CLC-7 is a member of the CLC family of chloride (Cl-) channels and chloride (Cl-)/proton (H+) transporters and is expressed in the lysosome and the resorption lacuna of osteoclasts. In the membranes of these acidic compartments, CLC-7 uses the large pH gradient to catalyze the uptake of two Cl- ions for each H+ released. Unique among mammalian CLC transporters, CLC-7 requires a β-subunit, osteopetrosis-associated transmembrane protein 1 (OSTM1), for transport activity. In this study, we present structures of the lysosomal Cl-/H+ exchanger CLC-7 alone and in complex with its obligatory β-subunit OSTM1.

Reconstruction of these particle images with two-fold symmetry imposed yielded a structure of CLC-7 in complex with OSTM1 at a resolution of 2.8 Å. The luminal domains of OSTM1 form a dimeric cap-like structure that covers the luminal surface of CLC-7 while the transmembrane helices pack against the periphery of the CLC-7 transmembrane domain. The luminal domain of OSTM1 is composed of two three-helix bundles. Connecting both within and between the helical bundles are five disulfide bonds that constrain the organization of the luminal domain. At the periphery of the luminal domain, non-protein densities were resolved extending from seven exposed asparagine residues (93, 128, 163, 184, 194, 263 and 274) on OSTM1. Because CLC-7 lacks any N-linked glycosylation sites, the glycosylation shell surrounding the rigid, disulfide-linked core of OSTM1 likely protects the luminal domain of CLC-7 from the harsh degradative environment of the lysosomal lumen. Binding of OSTM1 is accompanied by a bend in helix αB of CLC-7 at Gly149 that results in 9 Å shift of the luminal end of helix αB (measured at Cα of Glu168) toward helix αK. The interaction between transmembrane domains is largely mediated by the packing of hydrophobic residues, but polar interactions are formed between Tyr300 of OSTM1 and Glu416 and Trp503 of CLC-7 that may contribute to the specificity of the CLC-7/OSTM1 interaction. In the CLC-7/OSTM1 complex, the 25-residue linker between helices αK and αL forms two interactions with the luminal domain of OSTM1. In CLC-7/OSTM1, the side chain of Phe514 (conformation 1) narrows the constriction of this pathway to a minimum radius of 0.8 Å, which is too narrow to allow water molecules to enter the hydrophobic gap.

>[2x]MANVSKKVSWSGRDRDDEEAAPLLRRTARPGGGTPLLNGAGPGAARQSPRSALFRVGHMSSVELDDELLDPDMDPPHPFPKEIPHNEKLLSLKYESLDYDNSENQLFLEEERRINHTAFRTVEIKRWVICALIGILTGLVACFIDIVVENLAGLKYRVIKGNIDKFTEKGGLSFSLLLWATLNAAFVLVGSVIVAFIEPVAAGSGIPQIKCFLNGVKIPHVVRLKTLVIKVSGVILSVVGGLAVGKEGPMIHSGSVIAAGISQGRSTSLKRDFKIFEYFRRDTEKRDFVSAGAAAGVSAAFGAPVGGVLFSLEEGASFWNQFLTWRIFFASMISTFTLNFVLSIYHGNMWDLSSPGLINFGRFDSEKMAYTIHEIPVFIAMGVVGGVLGAVFNALNYWLTMFRIRYIHRPCLQVIEAVLVAAVTATVAFVLIYSSRDCQPLQGGSMSYPLQLFCADGEYNSMAAAFFNTPEKSVVSLFHDPPGSYNPLTLGLFTLVYFFLACWTYGLTVSAGVFIPSLLIGAAWGRLFGISLSYLTGAAIWADPGKYALMGAAAQLGGIVRMTLSLTVIMMEATSNVTYGFPIMLVLMTAKIVGDVFIEGLYDMHIQLQSVPFLHWEAPVTSHSLTAREVMSTPVTCLRRREKVGVIVDVLSDTASNHNGFPVVEHADDTQPARLQGLILRSQLIVLLKHKVFVERSNLGLVQRRLRLKDFRDAYPRFPPIQSIHVSQDERECTMDLSEFMNPSPYTVPQEASLPRVFKLFRALGLRHLVVVDNRNQVVGLVTRKDLARYRLGKRGLEELSLAQT;>MEPGPTAAQRRCSLPPWLPLGLLLWSGLALGALPFGSSPHRVFHDLLSEQQLLEVEDLSLSLLQGGGLGPLSLPPDLPDLDPECRELLLDFANSSAELTGCLVRSARPVRLCQTCYPLFQQVVSKMDNISRAAGNTSESQSCARSLLMADRMQIVVILSEFFNTTWQEANCANCLTNNSEELSNSTVYFLNLFNHTLTCFEHNLQGNAHSLLQTKNYSEVCKNCREAYKTLSSLYSEMQKMNELENKAEPGTHLCIDVEDAMNITRKLWSRTFNCSVPCSDTVPVIAVSVFILFLPVVFYLSSFLHSEQKKRKLILPKRLKSSTSFANIQENSN[2x]N-hydroxy-4-{[(2-hydroxyethyl)(phenylacetyl)amino]methyl}benzamide 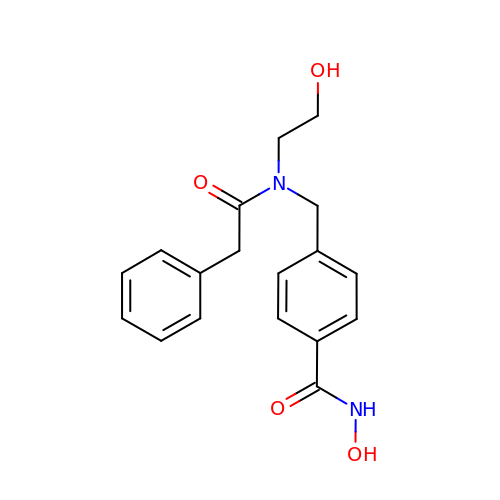| C18 H20 N2 O4 | GTFAUKGKYICUDS-UHFFFAOYSA-N> ADYQGKNVVIIGLGLTGLSCVDFFLARGVTPRVMDTRMTPPGLDKLPEAVERHTGSLNDEWLMAADLIVASPGIALAHPSLSAAADAGIEIVGDIELFCREAQAPIVAITGSNGKSTVTTLVGEMAKAAGVNVGVGGNIGLPALMLLDDECELYVLELSSFQLETTSSLQAVAATILNVTEDHMDRYPFGLQQYRAAKLRIYENAKVCVVNADDALTMPIRGADERCVSFGVNMGDYHLNHQQGETWLRVKGEKVLNVKEMKLSGQHNYTNALAALALADAAGLPRASSLK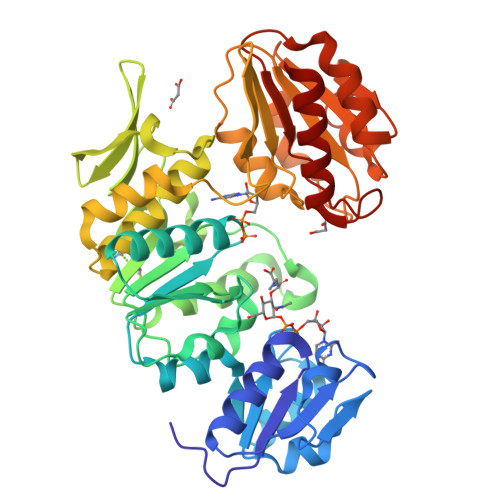ALTTFTGLPHRFEVVLEHNGVRWINDSKATNVGSTEAALNGLHVDGTLHLLLGGDGKSADFSPLARYLNGDNVRLYCFGRDGAQLAALRPEVAEQTETMEQAMRLLAPRVQPGDMVLLSPACASLDQFKNFEQRGNEFARLAKELGS> MNSSFPYFISPEQ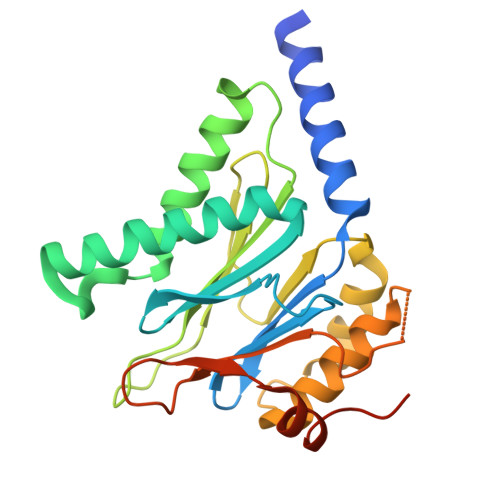AMRERSELARKGIARAKSVVALAYAGGVLFVAENPSRSLQKISELYDRVGFAAAGKFNEFDNLRRGGIQFADTRGYAYDRRDVTGRQLANVYAQTLGTIFTEQAKPYEVELCVAEVAHYGETKRPELYRITYDGSIADEPHFVVMGGTTEPIANALKESYAENASLTDALRIAVAALRAGSADTSGGDQPTLGVASLEVAVLDANRPRRAFRRITGSALQALLVDQESPQSDGESSG beta-D-mannopyranose | C6 H12 O6 | 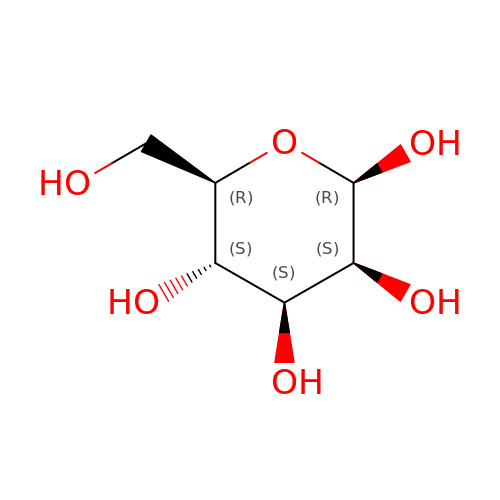WQZGKKKJIJFFOK-RWOPYEJCSA-N4-[6-(3,4,5-trimethoxyanilino)pyrazin-2-yl]benzamide 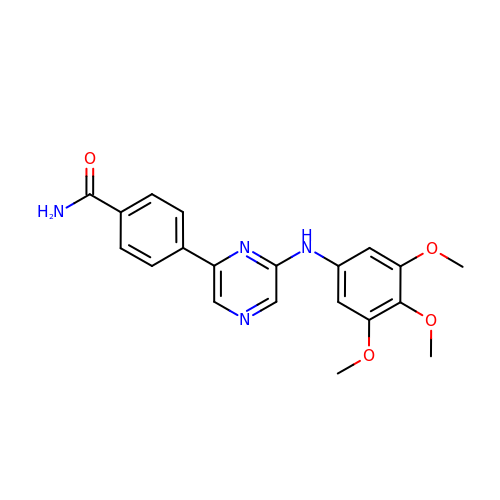| C20 H20 N4 O4 | LZLKDDDQYGMZTB-UHFFFAOYSA-N> MASSHHHHHHSSGLVPRGSHMSFDATAGALTVSLDTVDNTAQTANLSGTTTDVAPNEQVAITITDSAGNIVNAIATVGADGSYSLTGVDISSLVDGSLTVEASAQDRNGNALTDSANGALDATAGDLTVSVGTIDNTAQTVNLSGTTTDVAPNGQVAITMTDSAGNIVNATATVGADGSYSLTGVDISSLVDGDLTVEASAQDRNGNAVSDSANGTFDATAGDLTVSVDTVDSTAQTANLSGTTTDVALNSQVDLTVTDSAGNVVTATTTVGADGSYSLTGVDISSLVDGNLTVEATAQDRNGNAVSDSAAGSLDATTGALTVSLDTVDNAAQTVDLSGTTADVAPNSQVNVTITDSTGNVVNAITTVGADGSYSLTGVDISSLVDGDLTVE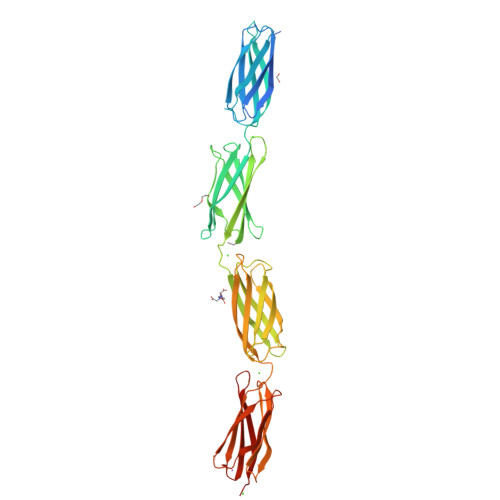ASAQGRNGNALTDSANGALDAT> VVTYTTLIDGLAKAGRLEEALQLFQEMKEKGVKPNVVTYTTLID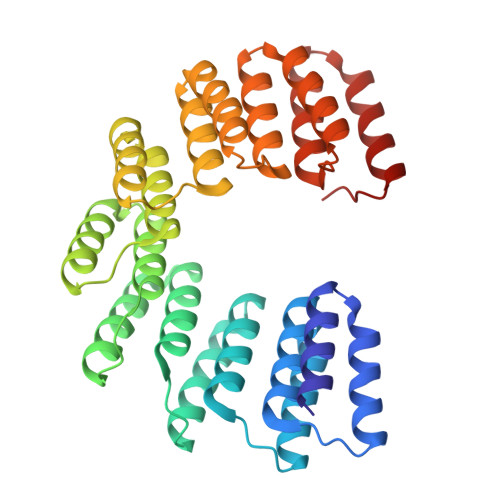GLAKAGRLEEALQLFQEMKEKGVKPNVVTYTTLIDGLAKAGRLEEALQLFQEMKEKGVKPNVVTYTTLIDGLAKAGRLEEALQLFQEMKEKGVKPNVVTYTTLIDGLAKAGRLEEALQLFEEMKEKGVKPNVVTYTTLIDGLAKAGRLEEALQLFQEMKEKGVKPNVVTYTTLIDGLAKAGRLEEALQLFEEMKEKGVKPNVVTYTTLIDGLAKAGRLEEALQLFEEMKEKGVKPNVVTYTTLIDGLAKAGRLEEALQLFQEMKEKGVKPN>KPNILIIMVDQLNGKLFPDGPADFLHAPNLKALAKRSARFHNNYTSSPLAAPARASFMAGQLPSRTRVYDNAAEYQSSIPTYAHHLRRAGYYTALSGKMHLVGPDQLHGFEERLTTDIYPADFGWTPDYRKPGERIDWWYHNLGSVTGAGVAEITNQMEYDDEVAFLANQKLYQLSRENDDESRRPWCLTVSFTHPHDPYVARRKFWDLYEDCEHLTPEVGAIPLDEQDPHSQRIMLSCDYQNFDVTEENVRRSRRAYFANISYLDEKVGELIDTL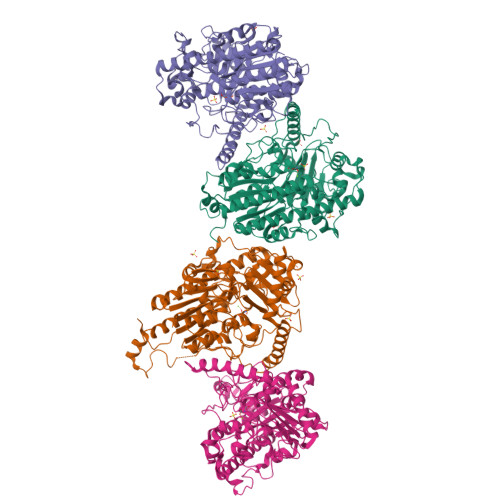TRTRMLDDTLILFCSDHGDMLGERGLWFKMNFFEGSARVPLMIAGPGIAPGLHLTPTSNLDVTPTLADLAGISLEEVRPWTDGVSLVPMVNGVERTEPVLMEYAAEASYAPLVAIREGKWKYVYCALDPEQLFDLEADPLELTNLAENPRGPVDQATLTAFRDMRAAHWDMEAFDAAVRESQARRWVVYEALRNGAYYPWDHQPLQKASERYMRNHMNLDTLEESKRYPRGE[4x]> MAHHHHHHTNPSESKFRLLENVNGVEVLTPLNHPPLQAWMPSIRQCVNKY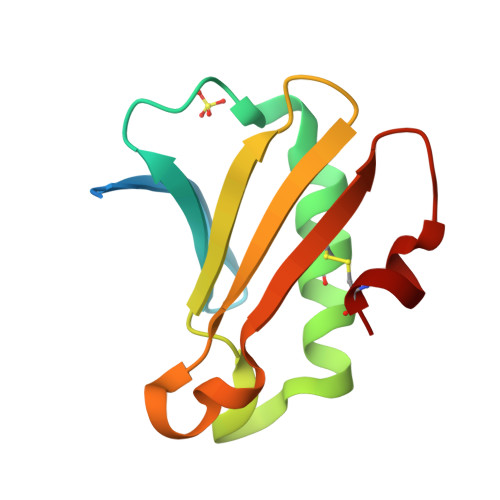AETHTGDSAPVKVIATGGQGNQLILNYIHTLPHSNENVTLRIFSEQNDLGSICK>MAHHHHHHMSLNTINPTETKAWAQLKEHFAETDFDLKQLFTEDKSRFSEFSIQKENLLFDFSKNLVDKKAFQLLLALAEECHLNDAIEKMFTGDLINQTENRAVLHTALRNFGEEKIVVNGKSIDEDVQRVLNQMKIFSEKIISGEHKGFSGKEITDVVNIGIGGSDLGPVMVCSALKHYRTRLNTHFVSNVDGNHIAEVVKNLNPETTLFIIASKTFTTQE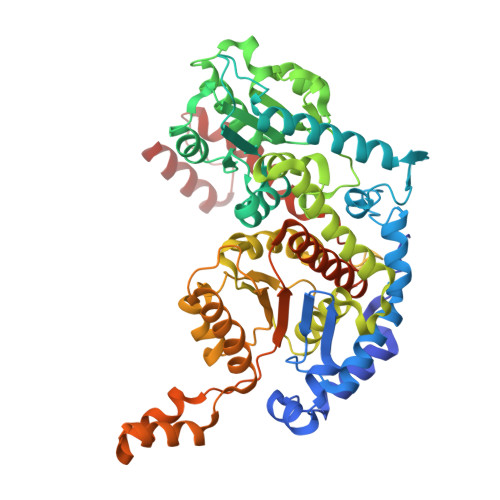TMTNALSAKEWFLKAGKEEDVAKHFVALSTNIEAVKNFGIAEENIFEFWDWVGGRYSLWSAIGLSIVLAVGYDNFEKLLRGAQDTDKHFRNTEFKNNIPVLMGVLGVWYRNFFDASSYAILPYSQYLDRFAAYLQQGDMESNGKSVDRNGEFVDYETGPIIWGEPGTNGQHAFYQLIHQGTELIPADFIAYAKANNNLSDHQDKLMSNFFAQTEALAFGKTKEQVITELKASGKNEEEIAFLTNFKTFTGNTPTNSFIFEELTPFTLGQLIAFYEHKIFVQGVIWNIFSFDQWGVELGKALANKILPELENTAEITSHDSSTNGLINFYKKHK[2x]> SSFKKILGLSSKSHKKSKKMGLPPPYDESSPMETQPSAPLSNDFFGMEDMDLYDKDSLRYEKFRFMLKMTVRSNKPFRSYDDVTAAVSQWDNSYIGMVGKRPFYKIIALIGSSHLQA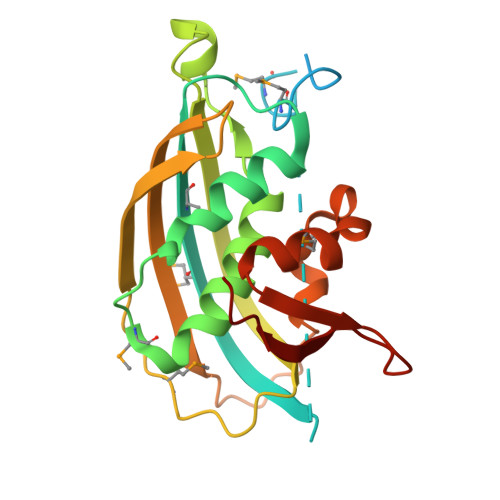TPAVLADLNQPEYYATLTGRCFLPHRLGLIPPMFNVSETFRKPFNIGIYKGTLDFTFTVSDDESNEKVPHVWEYMNPKYQSQIQKEGLKFGLILSKKATGTWVLDQLSPFK> MATSASSHLNKGIKQVYMALPQGDKVQAMYIWIDGTGEGLRCKTRTLDSEPKCIE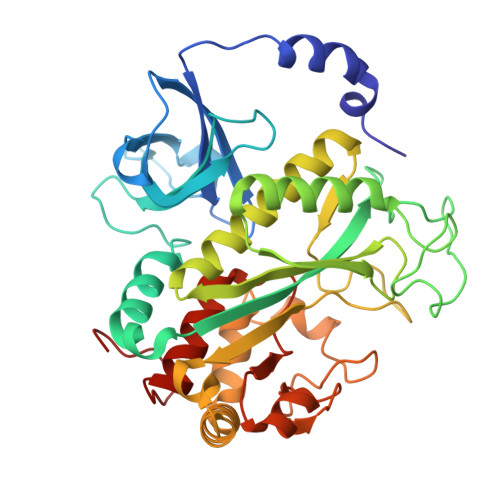ELPEWNFDGSSTFQSEGSNSDMYLVPAAMFRDPFRKDPNKLVFCEVFKYNRKPAETNLRHTCKRIMDMVSNQRPWFGMEQEYTLMGTDGHPFGWPSNGFPGPQGPYYCGVGADKAYGRDIVEAHYRACLYAGIKIGGTNAEVMPAQWEFQIGPCEGIDMGDHLWVARFILHRVCEDFGVIATFDPKPIPGNWNGAGCHTNFSTKAMREENGLKYIEEAIEKLSKRHQYHIRAYDPKGGLDNARRLTGFHETSNINDFSAGVANRGASIRIPRTVGQEKKGYFEDRRPSANCDPFAVTEALIRTCLLNETGDEPFQYKN>[3x]MGSSHHHHHHSQDPENLYFQGTGKFRYMPFSPAGTPFGFTDRRYLTMNEVGYVSTVKNSEQYSITVSFFDVGRFREYHFEDLFGYDLCFLNEKGTLFGQSKTGQIQYRPHDSIHSNWTKIIPLQAGERITSVAATPVRVIVGTSLGYFRSFNQFG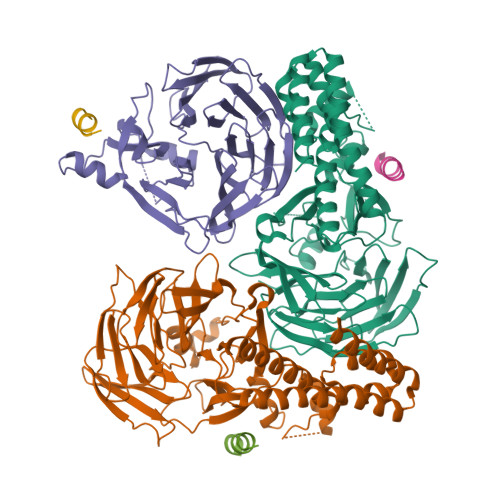VPFAVEKTSPIVALTAQNYRVFSVHYSQFHGLSYSLSELGTSSKRYYKRECPLPMSLPNINSDMKKDANLDYYNFNPMGIKSLFFSSYGDPCIFGSDNTLLLLSKWRSPEESKWLPILDSNMEIWKMSGGKETTDIHVWPLALAYDTLNCILVKGKHIWPEFPLPLPSEMEIRMPVFVKSKLLEENKAILNKKNEIGADTEAEEGEEDKEIQIPVSMAAEEEYLRSKVLSELLTDTLENDGEMYGNENEVLAALNGAYDKALLRLFASACSDQNVEKALSLAHELKQDRALTAAVKISERAELPSLVKKINNIREARYEQQLK;>[3x]SHAKDVKIQETIRKLNRFKPT Cthe_2751_is a 15.8 kDa singleton from an anaerobic, hyperthermophile Clostridium thermocellum, with an unknown function. Therefore, based on primary sequence analysis, Cthe_2751 is a non-Pfam singleton with an unknown function. Each monomer is made up of 8 α-helices arranged in a spiral pattern around a vertical axis that runs through the centre of the protein. The structure reveals an all α-helical topology similar to those observed for nucleic acid processing proteins.

Cthe_2751 crystallized as a dimer in 3 different crystal forms. Superimposition of the dimers crystallized in different space groups revealed no obvious differences in the position of the Cα atoms suggesting an identical mode of dimerization in all the 3 crystal forms. To find out if there is a difference in the packing arrangement of the dimers in the 3 crystal forms and to quantify it, a computer program was compiled and a calculation was performed to analyze the inter-dimer distances of 2 neighbouring dimers for all 3 space groups. As expected, the inter-dimer distance between 2 closest dimers in space groups C2221 and P4122 is relatively similar when compared to that of the distance between dimers of space groups P212121 and C2221 or P212121 and P4122, where there is almost no recognizable co-relationship. This result further supports the inferences of crystal packing analysis where we saw that the dimers rotate less than 3° along the C axes during the transformation from P4122 to C2221 resulting in only a minor change in crystal packing. A mathematical calculation performed on the dimers of Cthe_2751 crystallized in different space groups corroborated the findings of the crystal packing analysis of molecules packed in different space groups.

> MTSLRDLIPKHKFDNSTIDQLCKLIDNEIEPIIFDLLKWLQDYNWPIAKDILPVVVLHQSIAMPHILTILQGNDIMWKYWVIKLMIPYLIYPNKQLVKSELERLSSLEIINEDIREIVNLSKDYLHFYYP>[4x]GAIIFSAKDIFEQEFGREVRGYNKVEVDEFLDDVIKDYETYAALVKSLRQEIADLK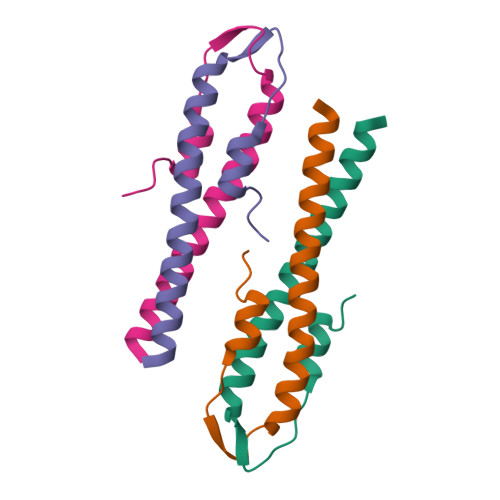EELTRK> GSHMEILWNEAKAFIAECYQELGKEEEVKDRLDSIKSEIDRTGSYVHTKEELEHGAKMAWRNSNRCIGRLFWNSLNVIDRRDVRTKEDVRDALFHHIETATNNGKIRPSITIFPPEEKGEKQVEIWNHQLIR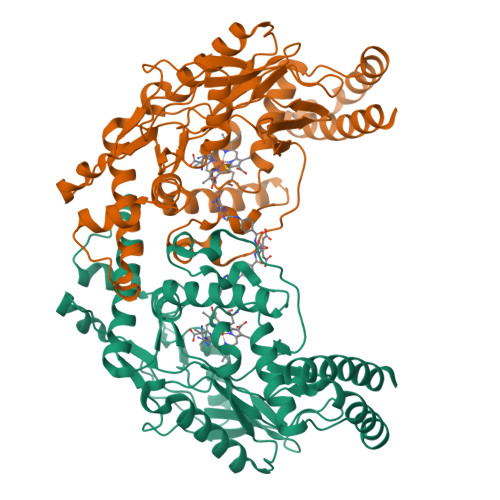YAGYESDGERIGDPASRSLTAACEQLGWRGERTDFDLLPLIFRMRGDEQPVWYELPRSLVIEVPITHPDIEAFSDLELKWYGVPIISDMKLEVGGIHYNAAPFNGWYMGTEIGARNLADEKRYDKLKKVASVIGISTNYNTDLWKDQALVELNKAVLYSYKKQGVSIVDHHTAASQFKRFEEQEEEAGRKLTGDWTWLIPPISPAATHIFHRSYDNSIVKPNYFYQDKPYE>GAMGSMNGIDDLLNINDRIKQVQNERNELASKLQNLKQSLASNDTEVALSEVIAQDIIEVGASVEGLEQLRAKYGDLQILNKLEKVAVQQTQMQAGVDKLDSFERQLDELAEQPPDQFTLDDVKALHSKLTSVFATVPQINNIDSQYAAYNKLKSKVTGKYNDVIIQRLATNWSNTFDQKLLEAQWDTQKFASTSVGLVKCLRENSTKLYQLSLLYLPLEEETQNGDSERPLSRSNNNQEPVLWNFKSLANNFNVRFTYHFHATSSSSKIETYFQFLNDYLAENLYKCINIFHDDCNGLTKPVIHEQFINYVLQPIRDKVRSTLFQNDLKTLIVLISQILATDKNLLNSFHYHGLGLVSLISDEVWEKWINYEVEMANRQFINITKNPEDFPKSSQNFVKLINKIYDYLEPFYDLDFDLLVRYKLMTCSLIFMNLTSSYLDYILTVDSLNETRTKEQELYQTMAKLQHVNFVYRKIKSLSSNFIFIQLTDIVNSTESKKYNSLFQNVENDYEKAMSTDMQNSIVHRIQKLLKETLRNYFKISTWSTLEMSVDENIGPSSVPSAELVNSINVLRRLINKLDSMD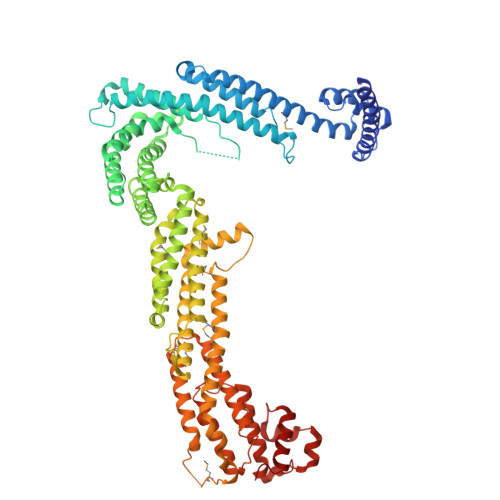IPLAISLKVKNELLNVIVNYFTESILKLNKFNQNGLNQFLHDFKSLSSILSLPSHATNYKCMSLHELVKILKLKYDPNNQQFLNPEYIKTGNFTSLKEAYSIKYLKDTKIQDALYRIIYGNIL[4x]> GSHMSAGNDRVRNLQSEVEGVKNIMTQNVERILARGENLDHLRNKTEDLEATSEHFKTTSQKVAR;> GSHM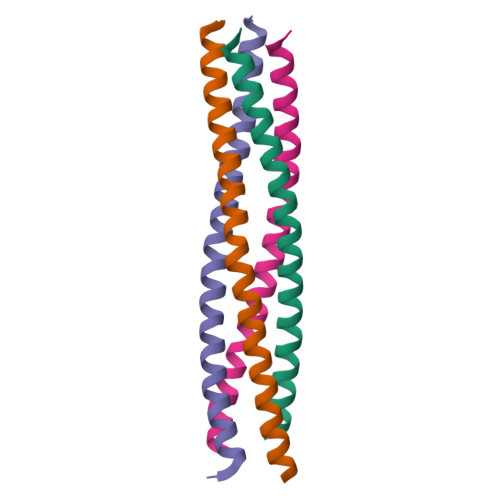HERESSIRQLEADIMDINEIFKDLGMMIHEQGDVIDSIEANVESAEVHVQQANQQLSRAAN;> GSHMNRATQSIERSHRIATETDQIGTEIIEELGEQRDQLERTKSRLVNTNENLSKSRKILRSMSR;> GSHMQEQDAGLDALSSIISRQKQMGQEIGNELDEQNEIIDDLANLVENTDEKLRTEARRVTLVDR> GQDIQ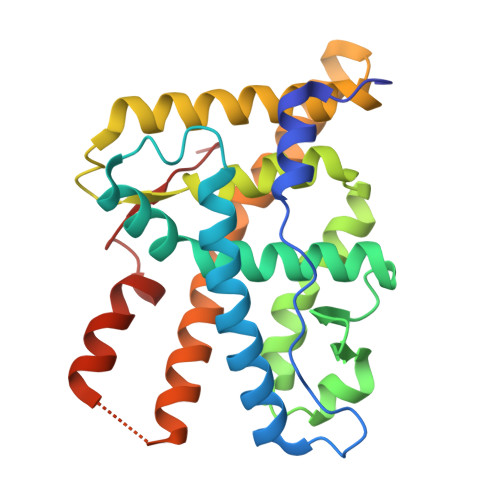LIPPLINLLMSIEPDVIYAGHDNTKPDTSSSLLTSLNQLGERQLLSVVKWSKSLPGFRNLHIDDQITLIQYSWMSLMVFGLGWRSYKHVSGQMLYFAPDLILNEQRMKESSFYSLCLTMWQIPQEFVKLQVSQEEFLCMKVLLLLNTIPLEGLRSQTQFEEMRSSYIRELIKAIGLRQKGVVSSSQRFYQLTKLLDNLHDLVKQLHLYCLNTFIQSRALSVEFPEMMSEVIAAQLPKILAGMVKPLLFHKK> SYFQSNMLWALLRQYVRPYRWLLAVVAVLQVISNMASLYLPTVNAAIIDDGVAKGDTARIVELGAVMLGVTALQVVCAVGAVFFGARAATGFGHDLRAAVFTHVTTFSAEEAGRFGAASLLTRTTNDVGHIQQLVQLTVTMLITAPIMSIGGIFMALHQDAGLSWLLLVSVPVLGLANYWIIRHLMPVFTRMQSLIDGINRVLRDQLSGI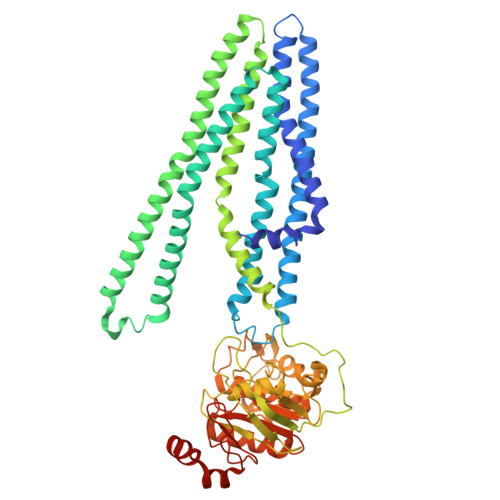RVIRAFAREPLERVRFAEANQTLSDSALEAGRWQALMLPVTTLVINVSSVALIWFGGLRIDAGQMQVGSLIAFLAYFMQILMAVLMATFMLVIFPRAAVCADRIGEVLSTQTAITNPADPVRPAAIAGDIGVHDATFCYPGADRPVLQDVSFTVPRGTTTAVVGSTGSGKSTLISLICRLYDVTSGSLRIDGVDVRDLDIEQLWSAIGLVPQRGYLFSGTVAENLRYGRADATDDEMWEALRVAAAADFVRAHPQGLDMPVAQGGINFSGGQRQRLAIARAVIRRPAIYLFDDAFSALDVHTDARVRDALREVAADATVVIVSQRISTVIEADQVVVIDDGRVVGIGTHDTLLADCPIYAEFAESQALTAGEPR Nucleosome assembly proteins (NAPs) are histone chaperones that are crucial for the shuttling and incorporation of histones into nucleosomes. The human malaria parasite P. falciparum contains two nucleosome assembly proteins, orthologs of eukaryotic NAPs, which have been previously termed PfNapL and PfNapS. PfNapL and PfNapS do not interact with each other and unlike PfNapL, PfNapS is able to deposit histones onto DNA. In the present study, the structural basis of nucleosome assembly activity in P. falciparum was addressed by determining and analysing the crystal structure of smaller NAP in the parasite called PfNapS.

A construct of PfNapS consisting residues 29-221 (molecular weight ~23 kDa) crystallized in orthorhombic space group P212121 with solvent content of 55% (the asymmetric unit contains three dimers of PfNapS). Crystal structure of PfNapS was determined using selenium-SAD (single anomalous dispersion) technique at 3.2 Å and refined using native data to 2.8 Å resolution. Four C-terminal residues (aa 218-221) were disordered as were regions 142-150 and 168-181. Each monomer of PfNapS contains domain I comprised of dimerization helix α2 (aa 33-73). The monomer also contains domain II, which is comprised of α-helices [α3 (aa 81-85), α4 (aa 99-102)] and a β sub-domain containing 4 anti-parallel β-strands (aa 106-158). In PfNapS, 23 residues of the dimerization helix α2 and four residues of α7 and α8 (which lie in domain II) contribute to dimer formation via hydrogen bonding and hydrophobic interactions (Asp32, Phe33, Ile36, Gln37, Ile40, Leu43, Asp44, Lys45, Cys47, Glu50, Gln51, Ile54, Gln55, Gln57, Tyr58, Lys61, Lys62, Leu65, Phe66, Lys68, Arg69, Ile72, Ile73 and His210, Pro212, Leu313, Leu217 respectively). Similar to PfNapL and other NAPs in the malaria parasite, PfNapS is also evolutionary distant from homologs in yeast and human. The length of the dimerization helix α2 varies in all the five proteins and PfNapS has the shortest such helix comprising of 41 residues. Also, the r.m.s.d. of PfNapS is lowest with hSET at 1.6 Å indicating high structural identity. Structural analysis reveals two free surface exposed cysteine residues (Cys47 and Cys154) in PfNapS dimer.

>[6x]FMQDFEDIQKDIEQLDIKCAHEQMNIQKQYDEKKKPLFEKRDEIIQKIPGFWANTLRKHPALSDIVPEDIDILNHLVKLDLKDNMDNNGSYKITFIFGEKAKEFMEPLTLVKHVTFDNNQEKVVECTRIKWKEGKNPIAAVTHNRSDLDNEIPKWSIFEWFTTDELQDKPDVGELIRREIWHNPLSYYLGLEE>PEIITPIITPFTKDNRIDKEKLKIHAENLIRKGIDKLFVNGTTGLGPSLSPEEKLENLKAVYDVTNKIIFQVGGLNLDDAIRLAKLSKDFDIVGIASYAPYYYPRMSEKHLVKYFKTLCEVSPHPVYLYNYPTATGKDIDAKVAKEIGCFTGVKDVIENIIHTLDYKRLNPNMLVYSGSDMLIATVASTGLDGNVALGSNYLPEVTVTIKKLAMERKIDEALKLQFLHDEVIEASRIFGSLSSNYVLTKYFQGYDLG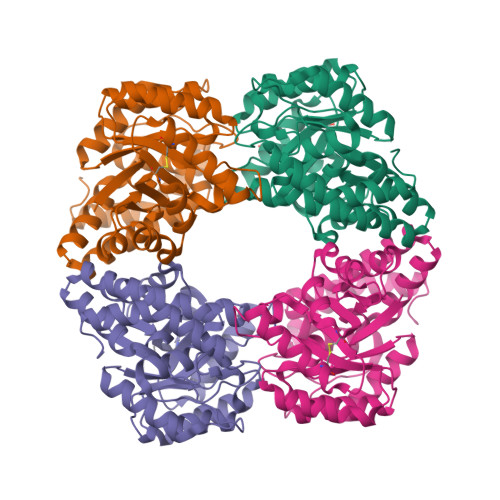YPRPPIFPLDDEEERQLIKKVEGIRAKLVELKILKE[4x]>[2x]MRDLYRNTNTFMIRTPIFSIDNYYEFFRKDGESDKIKDRLLEICNNSVFREAILVSSKSLYSTIIDFCDGKEIKKFDYFLQSIYKYLIRMSMRPTPFGLFSGVDFGKYAEETVISYENDNFKKFARPDLEWIIKIVKELEDNHYKNLTFKINDSIFIKGERALLIHSTDKEDNNRIGEISIRATKPFMRTYDLAKDGIEYNKLKYILIDEYSIEDESKIDNFLKQLIEREFLISNLRPPLTVLDQFDYLINEVKKAEIEIPLVDELTEIKEKLKLYNETPVGAGEETYLELYKKMESVANVKNILQVDMKLNLRDKKINKKIISDVNDLMNILLDLSMSIENPEPFLSKYKQEFIEKYGQDREISLLEMLDNDIGIGPPMNYERPRNNRSLDVSVNELLDNNVRDYFMEKYFQALKTNSRNIAIRDDEIKNLELQKIDYENIPDSLEINLLVKNKSEDNLSDEFQYYIGPNLGSTSAGKSFGRFSHMMSEPKKFFEELDERNIELIDSEEYVTCEISYLPSEVRNANVTRNIHSSEYEMSLFTNGSKDNLYRIKLNDIYIGLENNTFYAKSKTLNKKLLLTINNMLNPQTAPNAIRFLNDISLDEKKLWYKFVWSDVYKDFSYIPAIKYKNFVIMPETWKMNKINMKINKKTEFNEFKNQFNDYRIKYGVPQYVYITFADNRILLNLDDEQCVKILYHECKNSFNEIILNSYEEEGVNIVKESHKDYICELVIPLTKIKQETISDKVSARMLSSDISSLS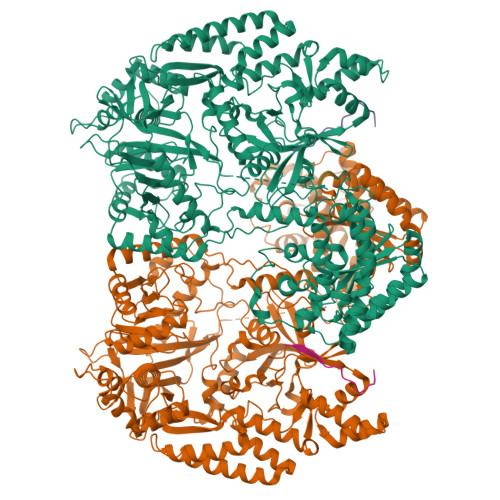KERVKDPFDEWLYIKLYGISSNVDDLIAYYISEFCNELVEEEIISKYFFMRYVDPEQHIRLRLNSSQEKLLMIYPKIREWLSMIRKKGLMTYFSIDSYDREIERYGGIELINIAEKVFFFDSIVTEDILRAKREGSFDFCDEIIGMISVVHYMESFGLPYAKQVEFLRSQVSSSEYREDFKQKRTEYMKLCNSNKDWEGLRESEEGNILIEILNKRRKIIEYYGNKVRENEEVSTDLSILDSIIHLNCNRMFGIDREFEKKVRALASHALYALKHFKS;>[2x]MGKLDDFDLDVKVKADTTKVGPAITSKSLCTPGCITGVLMCITQNSCVSCKSCIKC>MK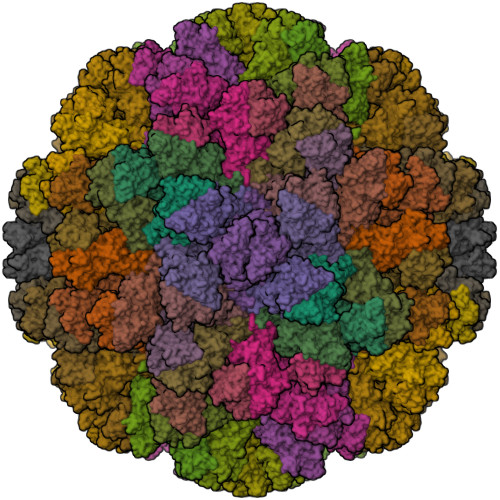MASSDASPSDGSTANLVPEVNNEVMALEPVVGAAIAAPVAGQQNVIDPWIRNNFVQAPGGEFTVSPRNAPGEILWSAPLGPDLNPYLSHLARMYNGYAGGFEVQVILAGNAFTAGKIIFAAVPPNFPTEGLSPSQVTMFPHIIVDVRQLEPVLIPLPDVRNNFYHYNQSNDPTIKLIAMLYTPLRANNAGDDVFTVSCRVLTRPSPDFDFIFLVPPTVESRTKPFTVPILTVEEMTNSRFPIPLEKLFTGPSGAFVVQPQNGRCTTDGVLLGTTQLSPVNICTFRGDVTHIAGTHDYTMNLASQNWNNYDPTEEIPAPLGTPDFVGKIQGVLTQTTRGDGSTRGHKATVSTGSVHFTPKLGSVQFTTDTNNDLETGQNTKFTPVGVVQDGNSAHQNEPQQWVLPNYSGRTGHNVHLAPAVAPTFPGEQLLFFRSTMPGCSGYPNMNLDCLLPQEWVLHFYQEAAPAQSDVALLRFVNPDTGRVLFECKLHKSGYVTVAHTGPHDLVIPPNGYFRFDSWVNQFYTLAPMGNGAGRRRAL[45x]Among them, levansucrases (sucrose: 2,6-β-d-fructan fructosyltransferase, EC 2.4.1.10) catalyze both sucrose hydrolysis, with the release of glucose and fructose, and levan synthesis. Levansucrase from Bacillus subtilis, Bacillus megaterium, Gluconacetobacter diazotrophicus, Erwinia amylovora, and Erwinia tasmaniensis was extensively purified, and their structure was described. ,− All of them display a single domain with a conserved five-bladed β-propeller topology. ,, Comparison of different levansucrases shows that the architecture of the central substrate-binding pocket is also conserved. In particular, the enzymatic mechanism of sucrose hydrolysis and levan synthesis involves the action of a catalytic triad including two aspartates, acting as a nucleophile and stabilizer, and a glutamate as a general acid/base catalyst. To gain insight into the binding mechanism, the X-ray crystal structures of the beta levansucrase isoform from P. syringae pv actinidiae (Psa) in its native form and in complex with TPIS were solved, confirming TPIS as a competitive inhibitor of levansucrases.

To provide a structural rationale for the multivalent effect observed in the enzyme inhibition by TPIS, we first determined the crystallographic structure of recombinant Lscβ in its apo form. Moreover, the first 16 amino acids of Lscβ do not have a counterpart in the EtLsc sequence. Nevertheless, this N-terminal region of Lscβ was not introduced in the model due to a lack of electron density. The active site is structurally conserved, with the catalytically essential residue Asp62, the nucleophile Asp219, and the acid/base catalyst Glu3038. Furthermore, the residues that compose the substrate-binding site are fully conserved with respect to EtLsc, and their side chains have similar conformations and orientations. Whereas, both enzymes present differences in this region compared to SacB: Ser164/Ala148, Arg360/His321, and Glu340/Gln301 (SacB/Lscβ numbering). These differences probably reflect the belonging of SacB to GH68 subfamily 1, instead of the subfamily 2. The two active sites, which are deeper compared to those of α-mannosidases and do not face one another in the dimer, are 55 Å apart, a much greater distance than that between two iminosugar-ending tails of TPIS (roughly 25 Å).

>[2x]SMSTSSSALSQLKNSPLAGNINYEPTVWSRADALKVNENDPTTTQPLVSADFPVMSDTVFIWDTMPLRELDGTVVSVNGWSVILTLTADRHPDDPQYLDANGRYDIKRDWEDRHGRARMCYWYSRTGKDWIFGGRVMAEGVSPTTREWAGTPILLNDKGDIDLYYTCVTPGAAIAKVRGRIVTSDQGVELKDFTQVKKLFEADGTYYQTEAQNSSWNFRDPSPFIDPNDGKLYMVFEGNVAGERGSHTVGAAELGPVPPGHEDVGGARFQVGCIGLAVAKDLSGEEWEILPPLVTAVGVNDQTERPHYIFQDGKYYLFTISHKFTYAEGLEGPDGVYGFVGEHLFGPYRPMNASGLVLGNPPEQPFQTYSHCVMPNGLVTSFIDSVPTDGEDYRIGGTEAPTVRIVLKGDRSFVQEEYDYGYIPAMKDVQLS>MDTPNKDDSIIRFSVSLQQNLLDELDNRIIKNGYSSRSELVRDMIREKLVEDNWAEDNPNDESKIAVLVVIYDHHQRELNQRMIDIQHASGTHVLCTTAIAMDEHNSLETIILQGNSF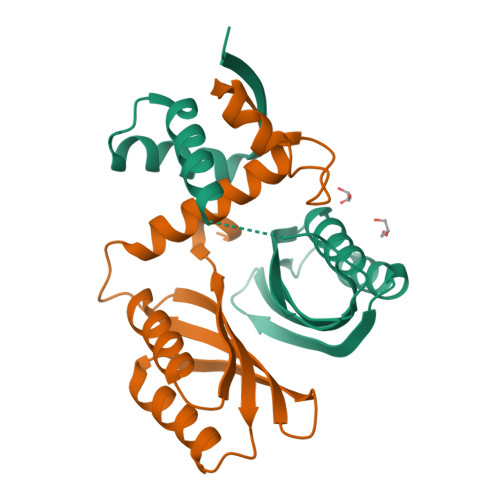EIQRLQLEIGGLRGVKFAKLTKASSFEYNE[2x]> GSMAEPLKEEDGEDGSAEP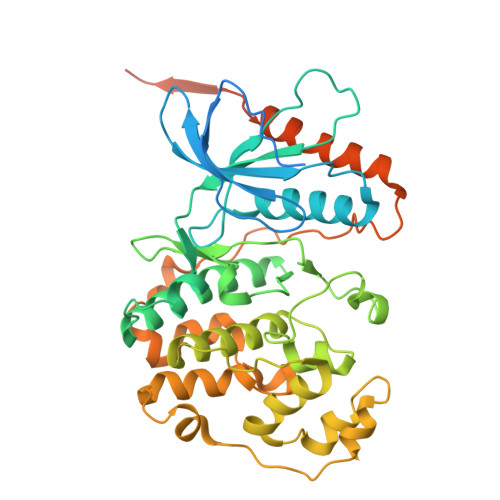PGPVKAEPAHTAASVAAKNLALLKARSFDVTFDVGDEYEIIETIGNGAYGVVSSARRRLTGQQVAIKKIPNAFDVVTNAKRTLRELKILKHFKHDNIIAIKDILRPTVPYGEFKSVYVVLDLMESDLHQIIHSSQPLTLEHVRYFLYQLLRGLKYMHSAQVIHRDLKPSNLLVNENCELKIGDFGMARGLCTSPAEHQYFMTEYVATRWYRAPELMLSLHEYTQAIDLWSVGCIFGEMLARRQLFPGKNYVHQLQLIMMVLGTPSPAVIQAVGAERVRAYIQSLPPRQPVPWETVYPGADRQALSLLGRMLRFEPSARISAAAALRHPFLAKYHDPDDEPDCAPPFDFAFDREALTRERIKEAIVAEIEDFHARREGIRQQIRFQPSLQPVASEPGCPDVEMPSPWAPSGDCAMSGRHHHHHH>[2x]MVSTAPYGAWQSPIDAALVASRSGRPACVGAVGDEVWWVAPRPAEAGRATLVRRRADGAEESALPAPWNVRNRVFEYSGFPWAGVPRPAGGPLLVFTHFGDQRLYAFEPDAPGGAVPRPLTPVSAVGGGLRWADPVLLPERGEVWCMAEEFTGEGPSDVRRFLAAVPLDGSAAADRSAVRELSDDAHRFVTGPRLSPDGRQAVWLAWDHPRMPWEGTELKTARVTEDGRFADTRTLLGGPEEAIAQAEWAPDGSLIVATDRTGWWNLHRVDPATGAATQLCRREEEFAGPLWTPGMRWFAPLANGLIAVVHGKGAAVLGILDPESGELVDAAGPWTEWAATLTVSGTRAVGVAASPRTAYEVVELDTVTGRARTIGARHTDPVDPAYYPEPQIRTFTAPDGREIHAHIYPPHSPDFTGPADELPPYVVMAHGGPTSRVPAVLDLDVAYFTSRGIGVADVNYGG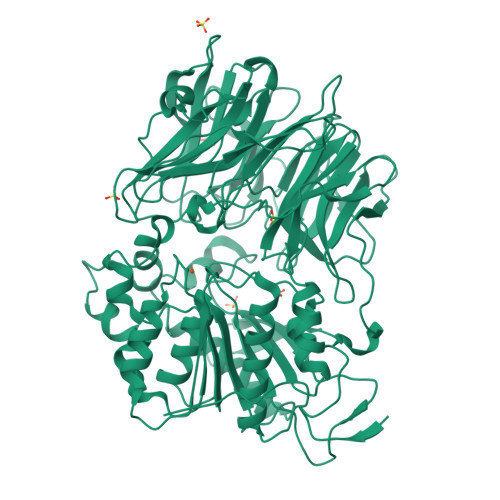STGYGRAYRERLRGRWGVVDVEDCAAVATALAEEGTADRARLAVRGGAAGGWTAASSLVSTDVYACGTVLYPVLDLLGWADGGTHDFESRYLDFLIGSFEEFPERYRDRAPLTRADRVRVPFLLLQGLEDPVCPPEQCDRFLEAVAGCGVPHAYLSFEGEGHGFRRKETMVRALEAELSLYAQVFGVEVAGVPLLKLGE;>PGG[2x]> SETDDLKWTERLPECPVYRPTKEEFEDPLTYLQKIFPEASKYGICKIVSPLTATVPAGAVLMKEKSNFKFTTRVQPLRLAEWDSDDKVTFFMSGRTYTFRDYEKMANKVFARRYCSGGSLPDSFLEKEFWKEIACGKTETVEYACDVDGSAFSSAPGDPLGSSKWNLNKVSRLPKSTLRLLETSIPGVTEPMLYIGMLFSMFAWHVEDHYLYSINYQHCGASKTWYGIPGSAALKFEKVVKECVYNDDILSTNGEDGAFDVLLGKTTIFPPKTLLDHNVPVYKAVQKPGEFVVTFPRAYHAGFSHGFNCGEAVNFAMGDWFPFGAIASCRYAHLNRVPLLPHEELICKEAMLLNSSSKSENLDLTPTELSGQRSIKTAFVHLIRFLHLARWSLMKSGLCTGLVSNTYGTIVCSLCKRDCYLAFINCECYSHPVCLRHDVKKLDLPCGTTHTLYLRDNIEDMEAAAMKFEKEDGVSDL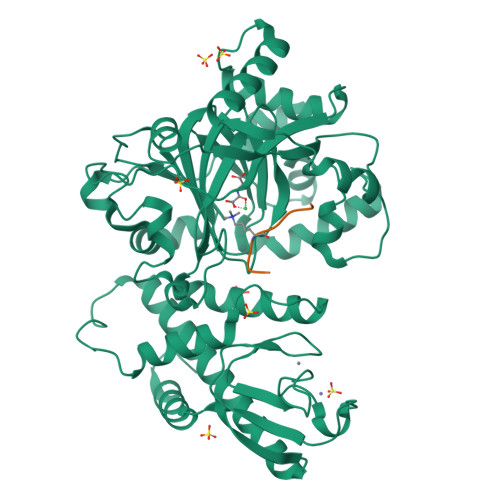ITTDEDLYKYPSS;> AARKSAPATGGV>GSHMMIVANMSSYPPRKKELVHSIQSLHAQVDKINLCLNEFEEIPEELDGFSKLNPVIPDKDYKDVGKFIFPCAKNDMIVLTDDDIIYPPDYVEKMLNFYNSFAIFNCIVGIHGCIYIDAFDGDQSKRKVFSFTQGLLRPRVVNQLGTGTVFLKADQLPSLKYMDGSQRFVDVR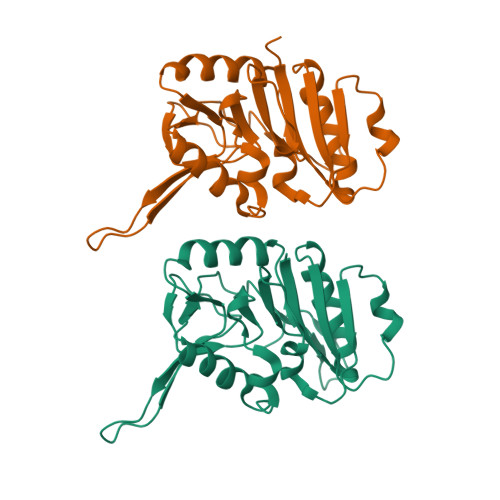FSRYMLENEIGMICVPREKNWLREVSSGSMEGLWNTFTKKWPLDIIKETQAIAGYSKLNLELVYNVEG[2x]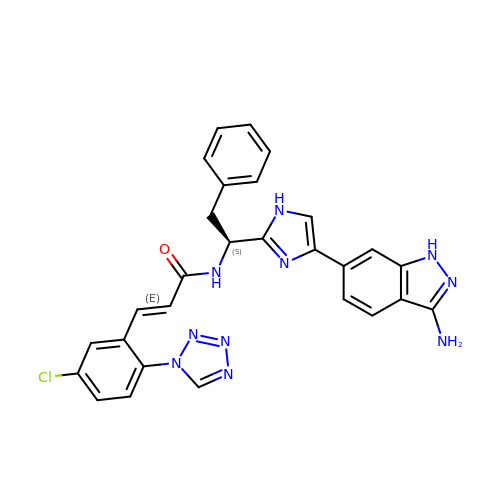(2E)-N-{(1S)-1-[4-(3-amino-1H-indazol-6-yl)-1H-imidazol-2-yl]-2-phenylethyl}-3-[5-chloro-2-(1H-tetrazol-1-yl)phenyl]prop-2-enamide | C28 H23 Cl N10 O | SSIRUUYXDLDNRC-BVRWQAIYSA-N> MHHHHHHAVRASEISRVYEAYPEKKATLYFLVLGFLALIVGSLFGPFQALNYGNVDAYPLLKRLLPFVQSYYQGLTLHGVLNAIV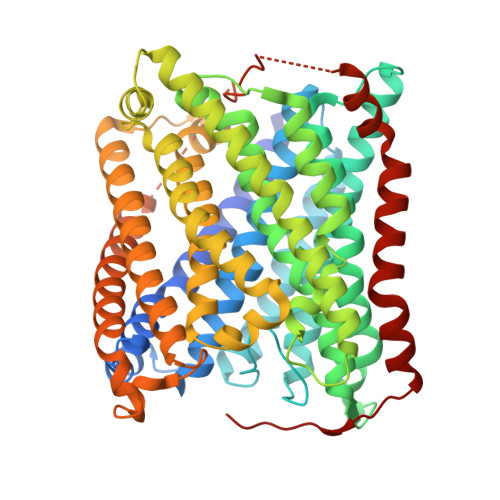FTQLFAQAIMVYLPARELNMRPNMGLMWLSWWMAFIGLVVAALPLLANEATVLWTFYPPLKGHWAFYLGASVFVLSTWVSIYIVLDLWRRWKAANPGKVTPLVTYMAVVFWLMWFLASLGLVLEAVLFLLPWSFGLVEGVDPLVARTLFWWFGHPIVYFWLLPAYAIIYTILPKQAGGKLVSDPMARLAFLLFLLLSTPVGFHHQFADPGIDPTWKMIHSVLTLFVAVPSLMTAFTVAASLEFAGRLRGGRGLFGWIRALPWDNPAFVAPVLGLLGFIPGGAGGIVNASFTLDYVVHNTAWVPGHFHLQVASLVTLTAMGSLYWLLPNLTGKPISDAQRRLGLAVVWLWFLGMMIMAVGLHWAGLLNVPRRAYIAQVPDAYPHAAVPMVFNVLAGIVLLVALLLFIYGLFSVLLSRERKPELAEAPLPFAEVISGPEDRRLVLAMDRIGFWFAVAAILVVLAYGPTLVQLFGHLNPVPGWRLW> SMYVIRDEWGNQIWICPGCNKPD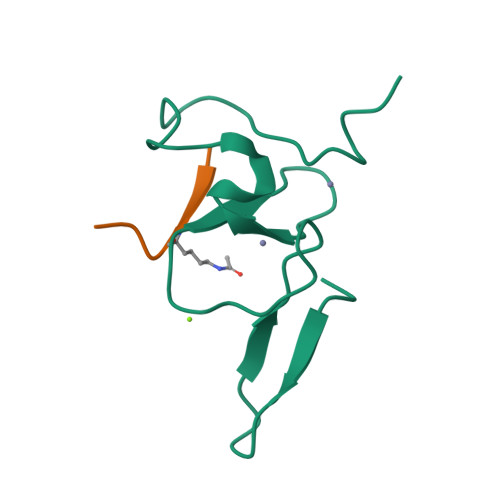DGSPMIGCDDCDDWYHWPCVGIMTAPPEEMQWFCPKCANK;> ARTKQTA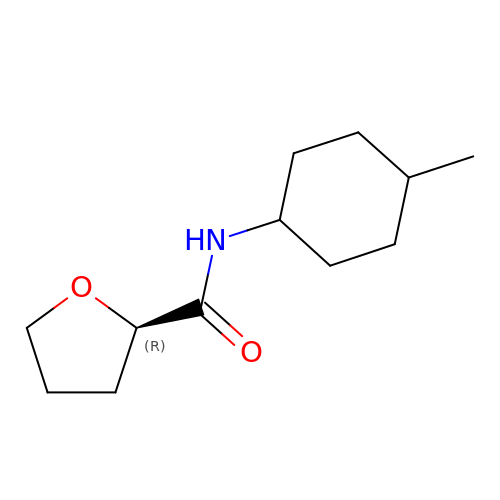(2R)-N-(trans-4-methylcyclohexyl)tetrahydrofuran-2-carboxamide | C12 H21 N O2 | CVLLQLWAZQCIEJ-GMTAPVOTSA-N>[8x]MAHHHHHHMEEAKHFIAGEWTLPAQLETIPVVDPSDGQPFATIARGTAPDIERAVAAARDAFAGPWGAASAAERGRVLMRLSARVTDSIEELAAIEARDTGKPLKQARADAAALARYFEFYAGAADKLHGETLPYQAGYTVLTVREPHGVTGHIVPW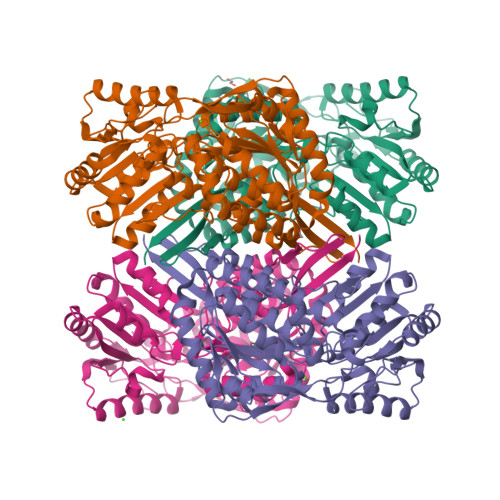NYPMQIFGRSVGAALAAGNACVVKPAEDACLSVLRVAELAAEAGLPAGALNIVTGYGHEAGAALARHPGIDHISFTGSPATGKLVTQMAAENHVPVTLELGGKSPQIVFADADLDAALPVLVSAIVQNGGQTCSAGSRVLIERAVYEPLVERLATAFNGLRVGPSRADLDCGPLINAKQQQRVWDFLSDAQHDGIPMAAHGQVVADAPESGFYQAPALLRDVPPSHRLAQEEVFGPVLAAMRFVDEDEAVALANGTPYGLVAGIWTRDGARQMRLARRLRAGQVFINNYGAGGGVELPFGGVGHSGHGREKGFEALYGFTALKTIAIRHG> MAHHHHHHMRFTLQREAFLKPLAQVVNVVERRQTLPVLANFLVQVQNGQLSLTGTDLEVEMVSRIAVEDAQDGETTIPARKLFEIIRALPDGSRITVSQTGDKITVQAGRSRFTLATLPSNDFPSVDEVEATERVAIGEATLKELIERTAFAMAQQDVRYYLNGLLFDLRGDALRTVATDGHRLALCETDLAKPSGSKRQIIVPRKGVTELQRLLESGDREIELEVGRSHVR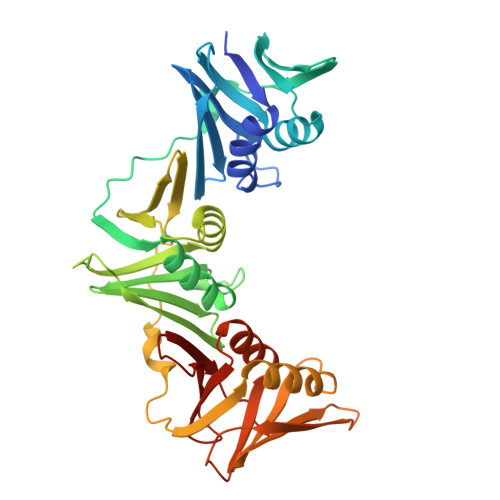VKRDDVTFTSKLIDGRFPDYEAVIPIGADREVKVDREALRASLQRAAILSNEKYRGIRVEVSPGNLKISAHNPEQEEAQEEIEADTTVSDLAIGFNVNYLLDALSALRDEEVIIQLRDSNSSALVRESSSEKSRHVVMPLRL>GFSNQVIQRGASGEDVIELQSRLKYNGFYTGKVDGVF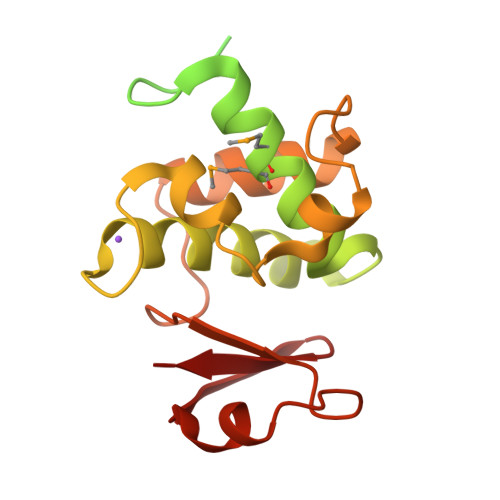GWGTYWALRNFQEKFGLPVDGLAGAKTKQMLVKATKYDKSTANKGNSGGTAQENKPSQNKGTNVPNGYSQNDIQMMANAVYGESRGEPYLGQVAVAAVILNRVTSASFPNTVSGVIFEPRAFTAVADGQIYLTPNETAKKAVLDAINGWDPTGNALYYFNPDTATSKWIWTRPQIKKIGKHIFCK[2x]>[2x]SNPFAHLAEPLDPVQPGKKFFNLNKLEDSRYGRLPFSIRVLLEAAIRNCDEFLVKKQDIENILHWNVTQHKNIEVPFKPARVILQDFTGVPAVVDFAAMRDAVKKLGGDPEKINPVCPADLVIDHSIQVDFNRRADSLQKNQDLEFERNRERFEFLKWGSQAFHNMRIIPPGSGIIHQVNLEYLA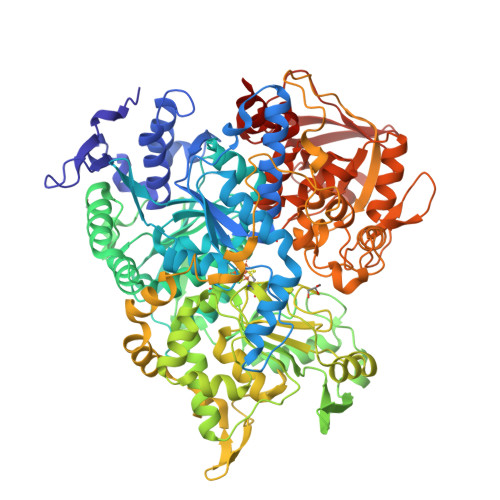RVVFDQDGYYYPDSLVGTDSHTTMIDGLGILGWGVGGIEAEAVMLGQPISMVLPQVIGYRLMGKPHPLVTSTDIVLTITKHLRQVGVVGKFVEFFGPGVAQLSIADRATIANMCPEYGATAAFFPVDEVSITYLVQTGRDEEKLKYIKKYLQAVGMFRDFNDPSQDPDFTQVVELDLKTVVPCCSGPKRPQDKVAVSDMKKDFESCLGAKQGFKGFQVAPEHHNDHKTFIYDNTEFTLAHGSVVIAAITSCTNTSNPSVMLGAGLLAKKAVDAGLNVMPYIKTSLSPGSGVVTYYLQESGVMPYLSQLGFDVVGYGCMTCIGNSGPLPEPVVEAITQGDLVAVGVLSGNRNFEGRVHPNTRANYLASPPLVIAYAIAGTIRIDFEKEPLGVNAKGQQVFLKDIWPTRDEIQAVERQYVIPGMFKEVYQKIETVNESWNALATPSDKLFFWNSKSTYIKSPPFFENLTLDLQPPKSIVDAYVLLNLGDSVTTDHISPAGNIARNSPAARYLTNRGLTPREFNSYGSRRGNDAVMARGTFANIRLLNRFLNKQAPQTIHLPSGEILDVFDAAERYQQAGLPLIVLAGKEYGAGSSRDWAAKGPFLLGIKAVLAESYERIHRSNLVGMGVIPLEYLPGENADALGLTGQERYTIIIPENLKPQMKVQVKLDTGKTFQAVMRFDTDVELTYFLNGGILNYMIRKMAK> DGDQCETSPCQNQGKCKDGLGEYTCTCLEGFEGKNCELFTRKLCSLDNGDCDQFCHEEQNSVVCSCARGYTLADNGKACIPTGPYPCGKQTLERRKRSVAQATSSSGEAPDSITWKPYDAADLDPTENPFDLLDFNQTQPERGDN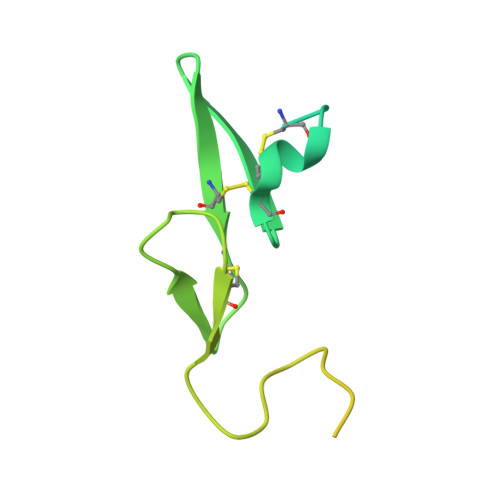NLTR>MRGSHHHHHHGSMDKNIIIGAMTALITPFKNGKVDEQSYARLIKRQIENGIDAVVPVGTTGESATLTNEEHRTCIEIAVETCKGTKVKVLAGAGSNATHEAVGLAKFAKEHGADGILSVAPYYNKPTQQGLYEHYKAIAQSVDIPVLLYNVPGRTGCEISTDTIIKLFRDCENIYGVKEASGNIDKCVDLLAHEPRMMLISGEDAINYPILSNGGKGVISVTSNLLPDMISALTHFALDENYKEAKKINDELYNINKILFCESNPIPIKTAMYLAGLIESLEFRLPLCSPSKENFAKIEEVMKKYKIKGF[6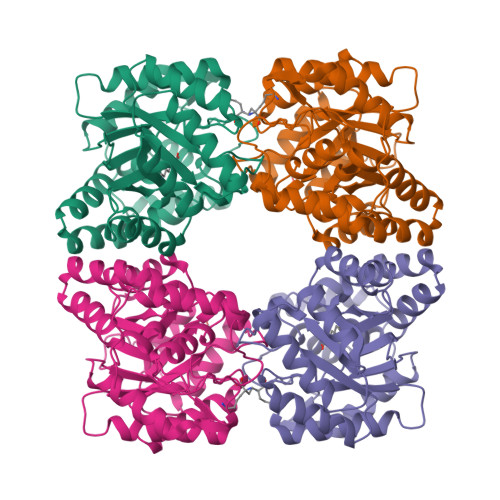x]> MSQPCPCGSADEYSLCCGRIVSGERVAPDPSHLMRSRYCAFVMKDADY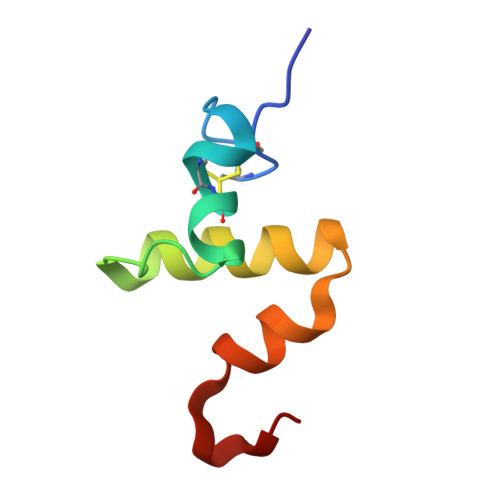LIKSWHPTCNAA N-[3-BENZYL-5-(4-HYDROXYPHENYL)PYRAZIN-2-YL]-2-(4-HYDROXYPHENYL)ACETAMIDE | C25 H21 N3 O3 | 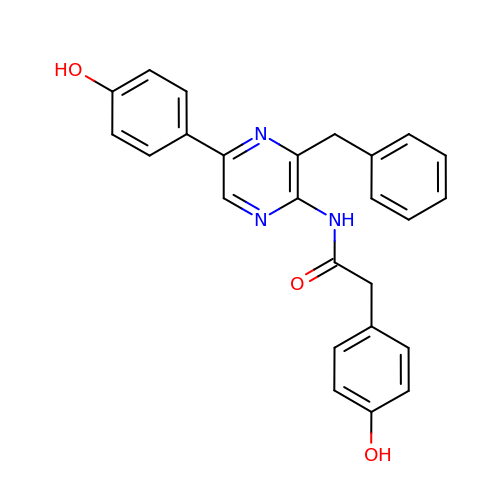CJIIERPDFZUYPI-UHFFFAOYSA-N> SVDLIGINVAGAEFTGGKLPGKHGTHYFFPPEGYFEYWSEQGIHTVR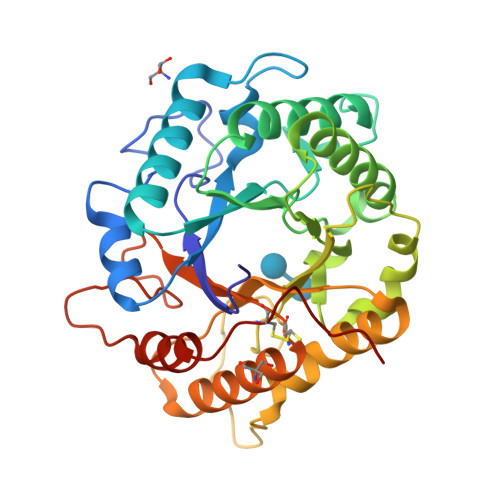FPLKWERLQPSLNAELDDVYASLVDDMLDQAKENDIKVILDVHNYARYRKKVIGTEDVPVSAYQDLMERIAKRWQGHDALFAYDIMNEPYGSADKLWPAAAQAGIDGVRKYDKKRPLLIEGASWSSAARWPRYADELLKLKDPADNMVFSAHVYIDEDASGSYKKGPGKDFEPMIGVKRVEPFVNWLKEHGKKGHIGEFGIPNDDERWLDAMDKLLAYLNENCIPINYWAAGPSWGNYKLSIEPKDGEKRPQVALLKKYAAKDNCSDFGPAKAE>MGAQSHSLEITSSVSAEKIFSGIVLDVDTVIPKAATGAYKSVEVKGDGGAGTVRIITL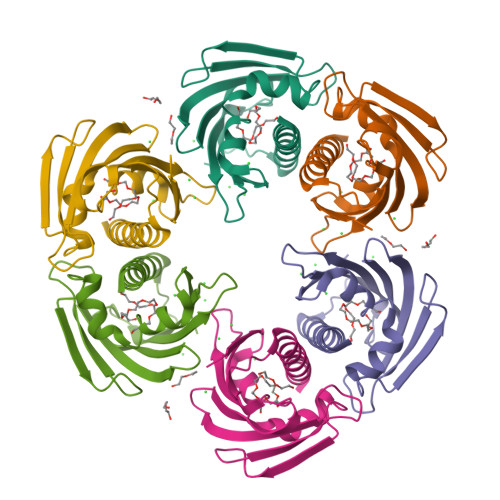PEGSPITTMTVRTDAVNKEALSYDSTVIDGDILLGFIESIETHMVVVPTADGGSITKTTAIFHTKGDAVVPEENIKFADAQNTALFKAIEAYLIAN[4x]> MPRVKSYTGGTINFKEIESHLVGSSATARKDAVEALIAYFDGSRTQSQTTFDDKAYHRLFEALFRCTLIEKEAYFNSKKSVKVTAAAAARLERCPEALRLAVRHGVTTIRRKTARAIIDHIVQVLPGPDGAYVMPLLAGYVKVLYEFLDNPASAENIAALSGEGWEVCVDFCIDVLSRFLELGDRESGSLSRASPAPGATARSGSVAGTQGSGEQIGTHVAVDVLSCLYMLCIAHNAPIQRKADRLPHVVIQLLQLRQMKIGELQKMAFATFNIVFQRMQAEDVALCKTLVKQVVPLLSHWWQPRALSRDAMLNSIRDEMLKTLYGTRLYIQALLREAADESFPQDVEELLDTLWCDYSRREERARLQLDDITFTNMLLPPDHPRTGIFSLRPHHTAGEQNWALLENLAILEAAYSKHGQQEQSQQNQQQPEIDQPRKRRKMSGRQNRVHQKLHSLDPAVRLSALQLIPFLTRHKKPSLEDVAETLEDLSKHVTAKQAIVASWAMLACSSLAIHEVSRHPSLSSSWKQLWQLAVRSLSLPPISRASCVLLNSILKANLIPRHELADDINQIVTTADISGPAILVDASLGLMLNLLRFRNNMFPNASQATSNHIIRWVFVRWSPAELTYASLHGTHATPYDLVNLLRACYGISPLVMAQPLRLFNGPIVLHWKEQAEMEPFIRYLLLLHEEEPDTTVTPAQQEEQLPESNSATDVAGSNASRRLALELFYPKVEELQELAESWQKRGGEGATPVSMERLRSMVLACLTGALLLPDLVNINSSLSRDLESAVFSIVDATLKVILNSPPSENLFGMILASSAPYIPHLIEPELIALKRERPHLLKFFGKLSEALYERSRRESSHRDDQVIDIDPDFEPQTSQKNTASKAKTLPRRDILLSYTPEAFYLETSLRIHFLDIIRLNDGEIGRIPEPIINQLAGLSGEQFLCCREFMREIFTSDAIVPLGGATTILETAGHIVSRYEYACCEVALCNCIDIMDSFINLWTDNHFDIAEMAGDLYHYLVKQSLPNNSMSAAAQIRLASLLLHLLEVKSEYASNLGLPSSQSTLLKILQDGPMKLKHYIGLEIPKLFGLYVLKTHDDIFVDVLEHLPSDPDVVEGLAFRLFVLAELACRWPTLLRRSIYHTFEIPGKITKISKSQSCVTHSALYAASCIKRIAQTLKLSGPQELFKLFAPQLLYTWLDNDSIQDIAYEIFGFSSLLDLLREAQTEAAAIMMMRGQEQEVCQLAQSLGLTPEKLVQQSFTKIIAYSIAHDISIAGGPDYVTGESRMRKILGKEEYLANIHLNFADIISTFFDIFDQEDPIEKAFRRDERFAYAAETLEEIKKLGHLPTALPPNQQPMFRAKYLPREIVHLCSRTQYEPENIWTPALVVFVARKLLKTIHPALGPLHACSVLRKIRVLICLAGDHAISGYPLEMLLHSLRVFVVDPECADDALGITQYLIKRGDEYLKRTPSFLAGYALSSLADLRVFLESSQSSTTQESQFKATKSKAQEFHAWFSKYLAAYDSPEFKDEGQKQAFRSITENAAHIRASGNAEKGTHESNLLLEILKDWGRENQLLNEPARDVALSMLCGVFNIPPSSRLDVIETDEDAIKNGAVVWKSCSSQRLGGEYLAWAGRVLGRSFAASGEVPEDLLRESQLQEYRRLSQGVGSSEEGLLNLIKSLTISGDCFTAGLAEAALRTIVSDAISDNDHDLLSACQESLPEPLLIASNWDPYRTPLSDQFKVDPPANTEVFSARALENPNWSQHLAIRLALSAPKIVTLRVLPPILSKVKGFAERAFPFVVHLVLAY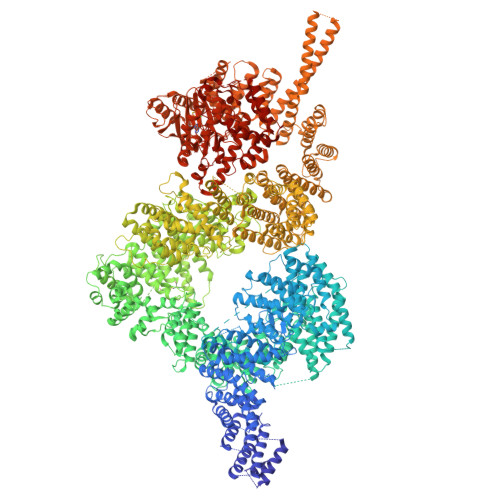QLDKQQSAKRELSESLQEWLNFTSEPAKENLKLLINTILYLRTQPLPGESSIADRAHWLDVNMASAAAAATRCGMYKVALLFAELAAESTRGSRRSSAARETDDSSDILLEIFENIDDPDAYYGLSQDASLSTVLARLEYENDGAKSLAFRGAQYDSHLRGRDLQSRQDCNALIKALSSLGLAGLSNSLLQSQQSIDGSSDSLDATFTTARKLEIWNLPAPVNSDSWAVTVYKAYQSMYQAQELDTVRSMVHDGLKNTVRHLSSGSLNTSVLRQQLGALAALTELDDILNVRDQSELQCTLATFEKRSKWMMSGRYADVSQILSCRETTLSMWSQRHNLRAAGLTSADARLVQIRGMLLSSDIFRFHRARQETLNLSTALSDLIPSCESLGLSVDAAIKMEAANALWDHGEMISSIRMLQAIDKDSSLKKQSVPLSRSDLLSKIGYQVSVARLESPDAIQKKYLEPALKELKGKIEGREAGQVFHQFAVFCDEQLQNPDSLEDLARLQNLKKGKDEEVAQLKALIASAKDSQLRNRYQSHLAKAKQWQELDQQELRRVEQTRSEFLKLCIENYLLSLAASDEHDNDALRFMALWLEKSEEEVANEVVKKWINKVPTRKFALLMNQLSSRLQDHNTLFQKLLIDLVYRICVDHPYHGMYHIWTGARTRVNKDDEVAVSRQRATDKIAKALSKNNKVSSIWPAIDQTSRVYHALAMDRDPTRYKSGQKVPIKNSPVGQNFLSTMSNNPIPPPTLQIEVSANLDYSHVPMIHKFAPEMAIASGVSAPKILTAIGTDGRKYKQLVKGGNDDLRQDAIMEQVFAAVSELLKLHRETRQRNLGIRTYKVLPLTSSSGLIEFVSNTIPLHEYLMPAHERYYPKDLKGSQCRKEIANAQTKNTETRIAVYRRVTERFHPVMRYFFMEYFPDPDEWFQKRTNYTRTTAAISMLGHVLGLGDRHGHNILLDHKTGEVVHIDLGVAFEMGRVLPVPELVPFRLTRDIVDGMGITKTEGVFRRCCEFTLDALREEAASIQTILDSLRHDTLYQWSISPVRMAKLQNAREVGGEDGGVGGGEDGEGGGVPKEKKQRPANEPSEADRAIEVVKKKLSKTLSVMATVNDLINQATSVSNLAVLYSGWAAYA> DTGERRCDPIRISMCQNLGYNVTKMPNLVGHELQTDAELQLTTFTPLIQYGCSSQLQFFLCSVYVPMCTEKINIPIGPCGGMCLSVKR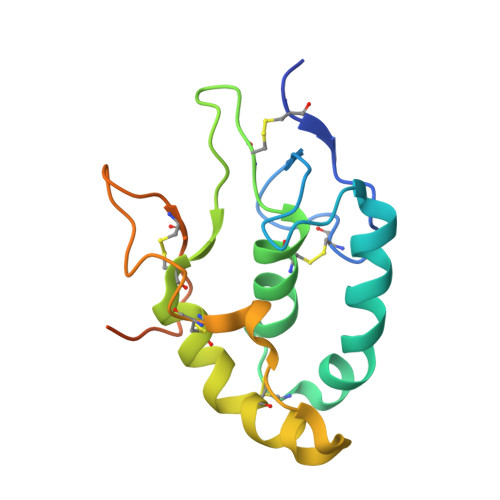RCEPVLKEFGFAWPESLNCSKFPPQNDHNHMCMEGPGDEEVPLPHKTPIQPGEGTLEVLFQ> MGSDKIHHHHHHMEIFGKTFREGRFVLKEKNFTVEFAVEKIHLGWKISGRVKGSPGRLEVLRTKAPEKVLVNNWQSWGPCRVVDAFSFKPPEIDPNWRYTASVVPDVLE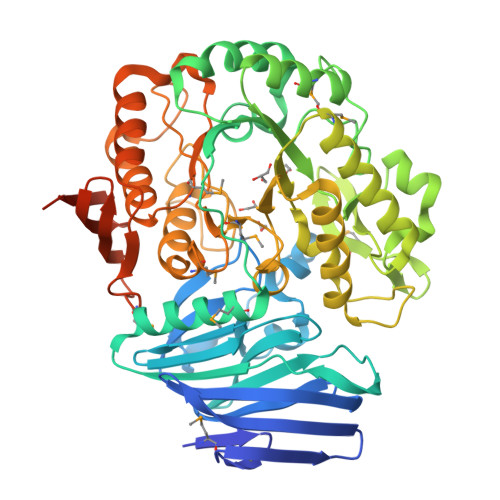RNLQSDYFVAEEGKVYGFLSSKIAHPFFAVEDGELVAYLEYFDVEFDDFVPLEPLVVLEDPNTPLLLEKYAELVGMENNARVPKHTPTGWCSWYHYFLDLTWEETLKNLKLAKNFPFEVFQIDDAYEKDIGDWLVTRGDFPSVEEMAKVIAENGFIPGIWTAPFSVSETSDVFNEHPDWVVKENGEPKMAYRNWNKKIYALDLSKDEVLNWLFDLFSSLRKMGYRYFKIDFLFAGAVPGERKKNITPIQAFRKGIETIRKAVGEDSFILGCGSPLLPAVGCVDGMRIGPDTAPFWGEHIEDNGAPAARWALRNAITRYFMHDRFWLNDPDCLILREEKTDLTQKEKELYSYTCGVLDNMIIESDDLSLVRDHGKKVLKETLELLGGRPRVQNIMSEDLRYEIVSSGTLSGNVKIVVDLNSREYHLEKEGKSSLKKRVVKREDGRNFYFYEEGERE>[2x]GYWGYQEFLDEFPEQRNLTNALSEAVRAQPVPLSKPTQRPIKISVVYPGQQVSDYWVRNIASFEKRLYKLNINYQLNQVFTRPNADIKQQSLSLMEALKSKSDYLIFTLDTTRHRKFVEHVLDSTNTKLILQNITTPVREWDKHQPFLYVGFDH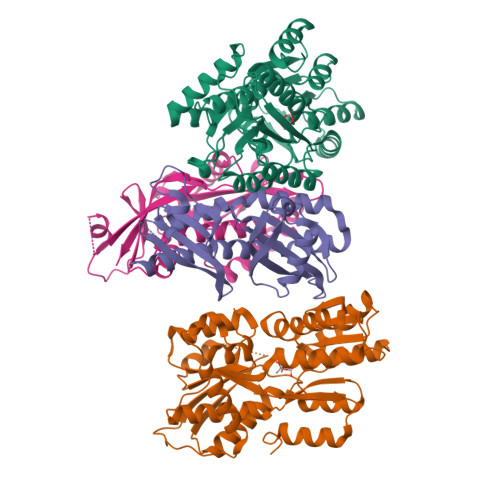AEGSRELATEFGKFFPKHTYYSVLYFSEGYISDVRGDTFIHQVNRDNNFELQSAYYTKATKQSGYDAAKASLAKHPDVDFIYACSTDVALGAVDALAELGREDIMINGWGGGSAELDAIQKGDLDITVMRMNDDTGIAMAEAIKWDLEDKPVPTVYSGDFEIVTKADSPERIEALKKRAFRYSDN;>GSKQQTSALIHNIFDSHFAAIQIHHDSNSKSEVIRDFYTDRDTDVLNFFFLSIDQSDPSHTPEFRFLTDHKGIIWDDGNAHFYGVNDLILDSLANRVSFSNNWYYINVMTSIGSRHMLVRRVPILDPSTGEVLGFSFNAVVLDNNFALMEKLKSESNVDNVVLVANSVPLANSLIGDEPYNVADVLQRKSSDKRLDKLLVIETPIVVNAVTTELCLLTVQD[2x]> MPLHMIPQVAHAMVRAAAAGRLTLYTRTRTETTNFDHAEYVTCGRYTICAFCLTTLAPHANVKTIQDSHACSRQPNEAIRSLVEVSDKAQTALVGSRT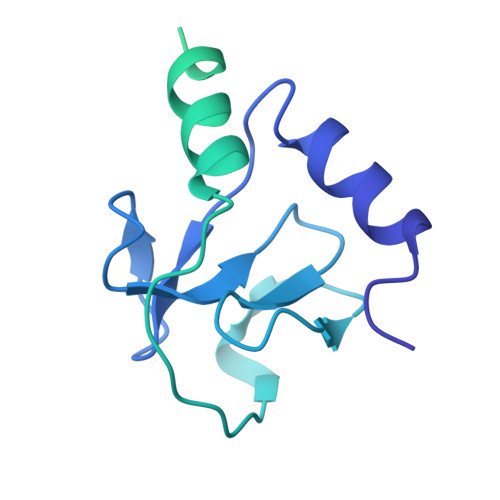VDYHELDVKAGFVAPTADETIAPSKDIVELPFRTCDLDDSSATACVRNHCQAGHDGVIHLPILSGDFKLPNEHPTKPLDDTHPHDKVLTRCPKTGLLLVHDTHAHATAVVATAATRAILMHDLLTSANADDGHQARSACYGPAFNNLTFACHSTCASDMAHFDCGQIVGLDLHVEPSD> MGYYRGEGTQDEEEGGASSDATEGHDEDDEIYEGEYQGIPRAESGGKGERMADGAPLAGVRGGLSDGEGPPGGRGEAQRRKEREELAQQYEAILRECGHGRFQWTLYFVLGLALMADGVEVFVVGFVLPSAEKDMCLSDSNKGMLGLIVYLGMMVGAFLWGGLADRLGRRQCLLISLSVNSVFAFFSSFVQGYGTFLFCRLLSGVGIGGSIPIVFSYFSEFLAQEKRGEHLSWLCMFWMIGGVYAAAMAWAIIPHYGWSFQMGSAYQFHSWRVFVLVCAFPSVFAIGALTTQPESPRFFLENGKHDEAWMVLKQVHDTNMRAKGHPERVFSVTHIKTIHQEDELIEIQSDTGTWYQRWGVRALSLGGQVWGNFLSCFGPEYRRITLMMMGVWFTMSFSYYGLTVWFPDMIRHLQAVDYASRTKVFPGERVEHVTFNFTLENQIHRGGQYFNDKFIGLRLKSVSFEDSLFEECYFEDVTSSNTFFRNCTFINTVFYNTDLFEYKFVNSRLINSTFLHNKEGCPLDVTGTGEGAYMVYFVSFLGTLAVLPGNIVSALLMDKIGRLRMLAGSSVMSCVSCFFLSFGNSESAMIALLCLFGGVSIASWNALDVLTVELYPS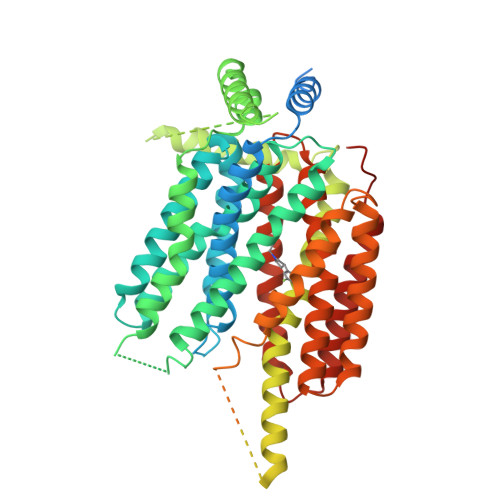DKRTTAFGFLNALCKLAAVLGISIFTSFVGITKAAPILFASAALALGSSLALKLPETRGQVLQLEVLFQ>MGLNFFRKAAPEVRTEPVAERKASVTGRIVAMASGAGRPVWGPRDTVSLMRTGFAGNPVGFRSVKLIAEATAAVPLICQDAERRYEIHPVLDLLRRPNAGQGRAELFEALIGQILLSGNGYLEAVCPEPGVPRELHVLRSDRMAVVPGADGWPVGYDYTVGGRKHRFDMTGHPDPICHIKSFHPTDDHYGLSPMQAAAVALDVHNAASAWSKALLDNAARPSGAIIYKGADGQGVLAPEQYERLIFEMETHHQGARNAGRPMLLEGGLDWKPMGFSPSDMEFHETKAAAAREIALAFGVPPMLIGIPGDATYANYAEANRAFYRLTVLPLLTRVSAALAWWLSGYLGAQIELKPDLDQVPALAVERDQLWARIGAAGFLSNSEKRVLLGLPPTAEG[2x];>[2x]MMLNEVTAVPGTALPVAEFRDHLRLGTGFADLGAEDAALLSYLRAAIAAIEGRTAKALISRGFRLALTAWRWGDMQTLPIAPVATVTALRLVDAAGVETPVAAGWRLVPDMARPRIEALGAMLPMIPTGGRVEIDFTAGFGASWSALPVDLAQAVFLLAAQYYELRHDGAAEGGAMPFGVMALIERWRTVRVLGGRP;> MSRPRLNRLLVLEEAVRVADGAGGHRLDWQAKGEVWAEVTAGSGSERAGEFVTLASVPFTIVVRAAPVGAARRPRPEQRFREGARIFRILAVAE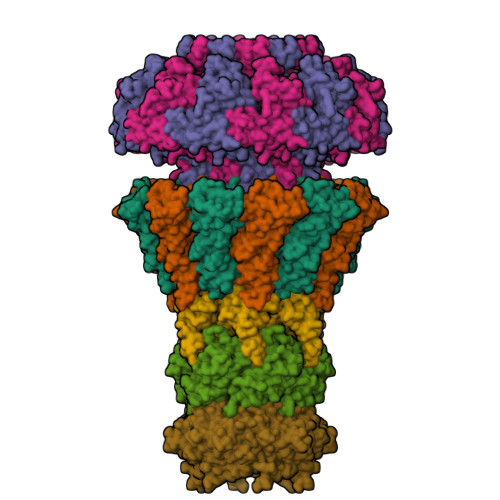RDREGHYLSCFAREEVVA;> MSYAVAGALQAAVYQQLRADAVLAALVGTAVYDAVPPGPLAGTYVSLGPEDVADASDKTGAGAVHDFVISVITDAAGFATAKAAAAAVSDALVGADLVLSRGRLVGLWFLRAKARRVEKADMRRIDLVFRARVEG;> MAAQNGKDLLIKLDLTGSGQFETIAGLRATRISFNAETVDVTSLESQGGWRELLGGAGVRSASISGAGVFKDADTDERARQIFFDGEVPEFQVIIPDFGIVQGPFMITSIDYAGSHNGEASYELAMASAGALSFTAI>MAIGEFMVSLPRMVYPQPKVLTPCRKDVLVVTPWLAPIVWEGTFNIDILNEQFRLQNTTIGLTVFAIKKYVAFLKLFLETAEKHFMVGHRVHYYVFTDQLAAVPRVTLGTGRQLS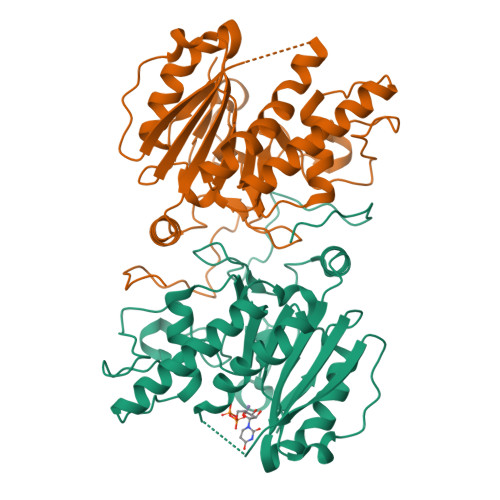VLEVGAYKRWQDVSMRRMEMISDFCERRFLSEVDYLVCVDVDMEFRDHVGVEILTPLFGTLHPSFYGSSREAFTYERRPQSQAYIPKDEGDFYYMGAFFGGSVQEVQRLTRACHQAMMVDQANGIEAVWHDESHLNKYLLRHKPTKVLSPEYLWDQQLLGWPAVLRKLRFTAVPMNHQAVRNP[4x]> MGMLEARELLCERDERTLFSGLSFTLNAGEWVQITGSNGAGKTTLLRLLTGLSRPDAGEVLWQGQPLHQVRDSYHQNLLWIGHQPGIKTRLTALENLHFY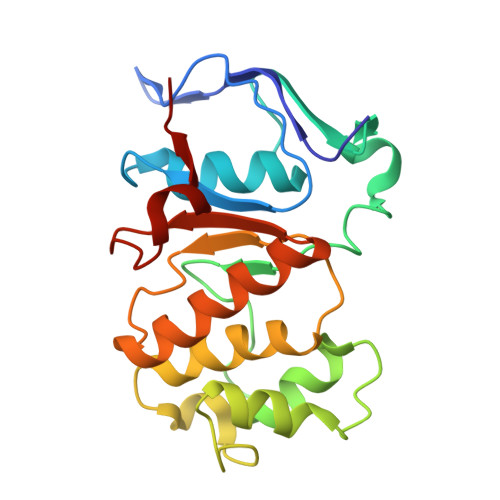HRDGDTAQCLEALAQAGLAGFEDIPVNQLSAGQQRRVALARLWLTRATLWILDEPFTAIDVNGVDRLTQRMAQHTEQGGIVILTTHQPLNVAESKIRRISLT>MTTADLILINNWHVVANVEDCKPGSITTARLLGVKLVLWRSQEQNSPIQVWQDYCPHRGVPLSMGEVANNTLVCPYHGWRYNQAGKCVQIPAHPDMVPPASAQA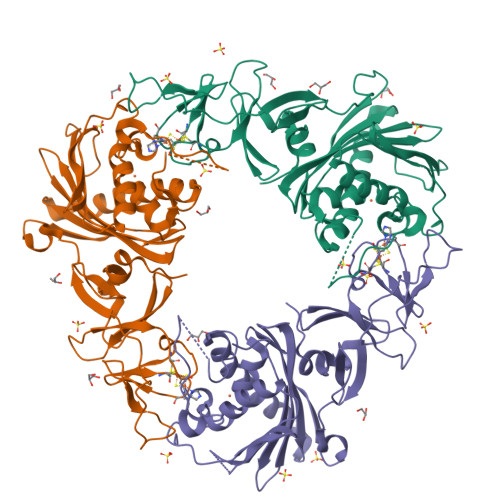KTYHCQERYGLVWVCLGNPVNDIPSFPEWDDPNYHKTYTKSYLIQASPFRVMDNSIDVSHFPFIHDGWLGDRNYTKVEDFEVKVDKDGLTMGKYQFQTSRIVSHIEDDSWVNWFRLSHPLCQYCVSESPEMRIVDLMTIAPIDEDNSVLRMLIMWNGSEMLESKMLTEYDETIEQDIRILHSQQPARLPLLAPKQINTQGLPQEIHVPSDRGTVAYRRWLKELGVTYGVC[3x]Vibrio dual lipases/transferases (VDLTs, e.g., VPA0226 of Vibrio parahaemolyticus, lec/VC_A0218 of Vibrio cholera, and VvPlpA of Vibrio vulnificus) are a class of virulence factors secreted by Vibrio pathogens to disrupt host membrane structures. VDLTs contain an N-terminal domain (NTD) of unknown function and a C-terminal catalytic domain belonging to the SGNH/GDSL hydrolase family, which is named after the four characteristic catalytic residues (Ser, Gly, Asn, and His). Therefore, VDLTs are enzymes with unusual dual substrate and catalytic promiscuity, which could benefit pathogens in handling diverse host lipid molecules in a proper manner. Crystal structures of the VDLT from Vibrio alginolyticus (ValDLT) and its fatty acid complexes were solved, revealing prominent structural flexibility.

The apo ValDLT was crystallized in the P21 space group with two protein monomers in one asymmetric unit. However, unlike the occluded active site in VvPlpA, the active site in ValDLT is readily accessible from the solvent region. A polyethylene glycol (PEG) molecule derived from the crystallization buffer could be modeled in the substrate-binding pocket of each monomer. Nevertheless, the superposition also identified conformational heterogeneity in both terminal regions and some additional regions, such as loopβ3−β4 (81WWSSVSFKNM90) and loopβ8−α5 (202VGGAAGENQYIALT215), indicating flexibility in these structural segments. Notably, loopβ8−α5 is located at the opening of the substrate-binding pocket. It exhibits a defined conformation in monomer B; however, in monomer A, most of it (residues 204 to 214) is completely disordered, lacking defined electron density to trace. In comparison, ValDLT contains a canonical Ser−His−Asp catalytic triad composed of residues S153, H393 and D390, with the oxyanion hole contributed by the main-chain NH groups of S153 and G204 and the side-chain amide group of N248. In monomer A, the oxyanion hole is ambiguously defined, as G204 is located at the disordered region of loopβ8−α5. In monomer B, the same region is in an ordered conformation that brings G204 into a proper oxyanion-hole forming position, due to a Mg2+ cation that bridges E208 and D263. Furthermore, another oxyanion hole residue, N248 in monomer B, differs in the side-chain conformation from that of monomer A. Unlike those in VvPlpA and monomer A, the oxyanion hole in monomer B appears to be well-formed, with a water molecule occupying the putative oxyanion hole position, stabilized by the hydrogen bonds from all three oxyanion hole residues, S153, G204 and N248.

>[2x]MGMMKKTITLLTALLPLASAIAEEPTLSPAMVSAAEVVSAQENQTYTYVRCWYRTSHSKDDAATDWKWAKNQDGSDFTIDGYWWSSVSFKNMFYTNTSQNVIRQRCEETLDLANENADITFFAADNRYSYNHTIWSNDAAMQPDQINKVVALGDSLSDTGNIFNASQWRFPNPNSWFLGHFSNGFVWTEYVAKAKNLPLYNWAVGGAAGENQYIALTGVGEQVSSYLTYTKLAKNYNPANTLFTLEFGLNDFMNYNRSVPEVKADYAEALIRLTDAGAKNFMLMTLPDATKAPQFKYSTQEEIETIRAKVLKMNEFIKAQAMYYKAQGYNIALFDTHALFEKLTSAPEEHGFVNASDPCLDINRSSSVDYMYTHSLRSECAASGADKFVFWDVTHPTTATHRYVAEKMLESSNNLEEFRFHHHHHH> SSVKRQSTARTRSFTETNRRTPSVQSKHEFWEDPDDGSDSENEYEGEEEDGIGNDLDNESDWEDDSRVQKLTTTDNYEEELAKEVEQLLEPEERVILQQNEKPNLKMISTKSWKPLQTLALSMQIQLMDNLIENGLDIDDVDKDNQTALHKAIIGKKEAVISHLLRKGANPHLQDRDGAAPIHYAVQVGALQTVKLLFKYNVDVNVADNEGWTPLHIAVQSRNRDITKILLTNGADKTRRTKDGKLALDLALCFGRDFKSYDLVKLLKIMPTGDI;> SLSYSSQTSILPDAGDDFIVGDCLVYEDGVFEDPYLDKEVTQVAKQERKKNRRGGAKRLDESEIEPENLVPEEWRDIQAEVNLTKKDKRKIAQEMEFGVRVEKKRQGLIPLRKVDLNDFLTYKEAKLAQLRPVILDKPGNFSDDSGASSDGETAVSSPSERVAPKNPRWAVYGKGFDHVAKFFNSDKYDPSDKKSDGPRKLLSKEEKFMLNSRNPDLAVATSKKWLPLHTLAACGEFYLVDSLLKHNLDINATDVGGLTVLHRAIIGKKQAITNYLLRESANPF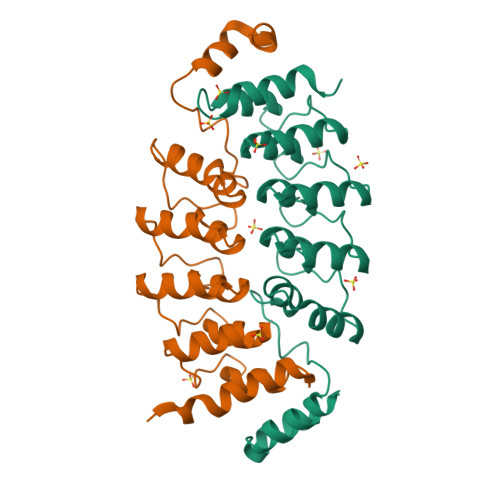VLDDEGATLMHYAVQTASAPTIKLLLLYNADINAQDRDGWTPLHVAVQARRSDIVKLLLIKGADIEVKNKDGLTPLGLCLYLGREIRTYEVMKLLKEFPLSRHKKRLVTTDEDIE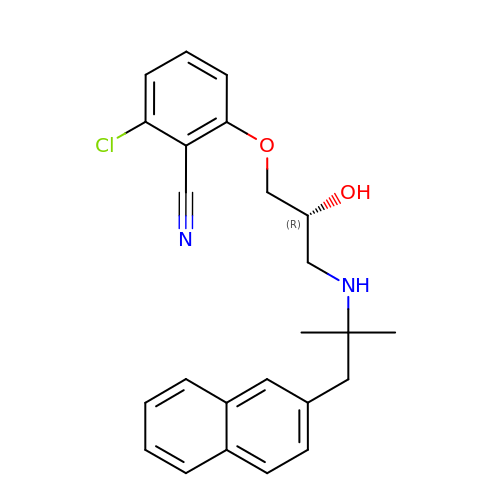2-chloro-6-[(2R)-2-hydroxy-3-{[2-methyl-1-(naphthalen-2-yl)propan-2-yl]amino}propoxy]benzonitrile | C24 H25 Cl N2 O2 | PZUJQWHTIRWCID-HXUWFJFHSA-N> LTGYTLSEVVPLKDV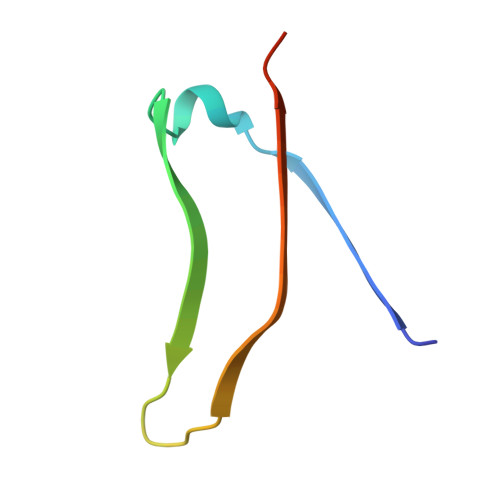VPEWVRIGFSATTGAEYATHEVLSWTFLSELTGPSN> VALFPVALF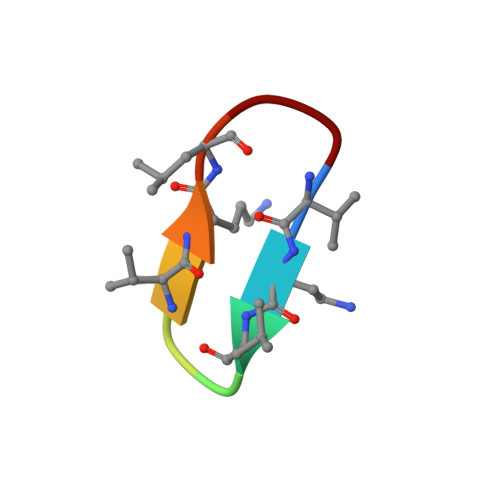P>[4x]VMFIDGKWINREDMDVINPYSLEVIKKIPALSREEAKEAIDTAEKYKEVMKNLPITKRYNILMNIAKQIKEKK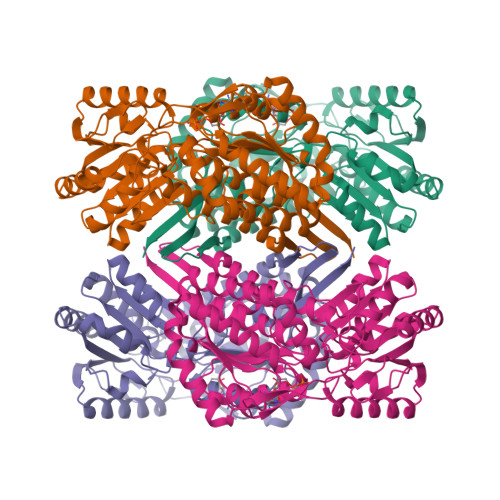EELAKILAIDAGKPIKQARVEVERSIGTFKLAAFYVKEHRDEVIPSDDRLIFTRREPVGIVGAITPFNFPLNLSAHKIAPAIATGNVIVHHPSSKAPLVCIELAKIIENALKKYNVPLGVYNLLTGAGEVVGDEIVVNEKVNMISFTGSSKVGELITKKAGFKKIALELGGVNPNIVLKDADLNKAVNALIKGSFIYAGQVCISVGMILVDESIADKFIEMFVNKAKVLNVGNPLDEKTDVGPLISVEHAEWVEKVVEKAIDEGGKLLLGGKRDKALFYPTILEVDRDNILCKTETFAPVIPIIRTNEEEMIDIANSTEYGLHSAIFTNDINKSLKFAENLEFGGVVINDSSLFRQDNMPFGGVKKSGLGREGVKYAMEEMSNIKTIIISKAENLYFQSHHHHHHWSHPQFEK>MVHLNKTIQEGDNPDLTAERLTA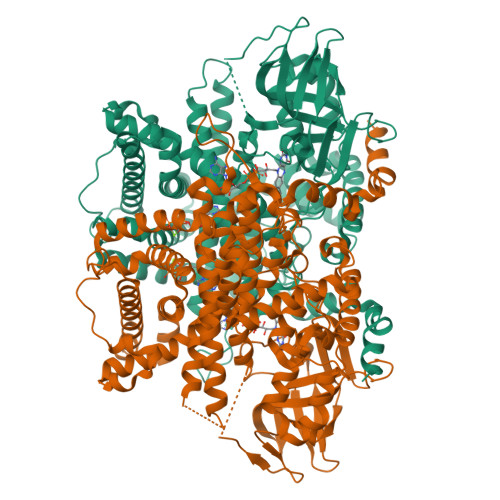TFDTHAMAAQIYGGEMRARRRREITAKLAEIPELHDSMPLPYMTREEKIMESARKLTVLTQRMSEIIDPTDAGELYHLNNEVLGIEGNPMALHGVMFIPALNAQASDEQQAKWLIRALRREIIGTYAQTEMGHGTNLQNLETTATYDIGTQEFVLHTPKITALKWWPGNLGKSSNYAVVVAHMYIKGKNFGPHTFMVPLRDEKTHKPLPGITIGDIGPKMAYNIVDNGFLGFNNYRIPRTNLLMRHTKVEADGTYIKPPHAKINYSAMVHVRSYMLTGQAIMLSYALNIATRYSAVRRQGQIDKNEPEVKVLEYQTQQHRLFPFIARAYAFQFAGAETVKLYERVLKEMKSGNVSLMADLHALTSGLKSVVTHQTGEGIEQARMACGGHGYSMASYISEIYGVAIGGCTYAGENMVMLLQLARYLVKSAALVKSGKASQLGPLVAYLGARSEPTSLIDRVPNGGITEYIKTFQHIAKRQTLKAANKFFGLMENGEKREIAWNKSSVELNRASRLHTRLFIVEAFARRVNEIGDITIKEALSDLLHLHVNYELLDVATYALEDGFMSSTQLDYVRDQLYFYLQKIRPNAVSLLDSWEFSDRELRSVLGRRDGHVYENLFKWAKESPLNKTDVLPSVDTYLKPMMEKARQSKLHHHHHHHHHH[8x]>[6x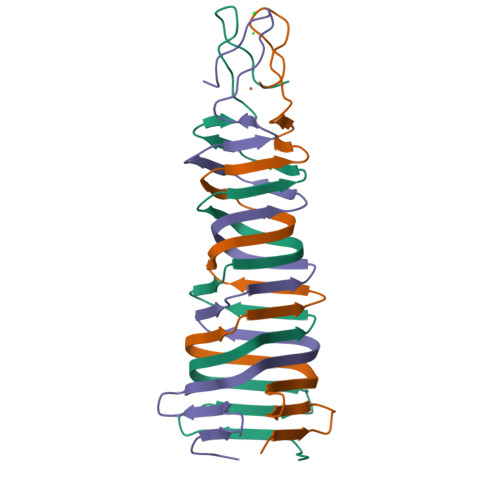]MHHHHHHHHSGDNPSPSVSADALHIRFPDGAVIEYEPETSALTVSGIKTASVTASGSVTATVPVVMVKASTRVTLDTPEVVCTNRLITGTLEVQKGGTMRGNIEHTGGELSSNGKVLHTHKHPGDSGGTTGSPL>VSEDLRSRIEVLKRKVIEKVQHIQLLQKNVRAQLVDMKRLEVDIDIKIRSCRGSCSRALAREVDLKDYEDQQKQLEQVIAKDLLPSR[2x];>DNENVVNEYSSELEKHQLYIDETVNSNIPTNLRVLRSILENLRSKIQKLESDVSAQMEYCRTPCTVSCNIPVVSGKECEEIIRKGGETSEMYLIQPDSSVKPYRVYCDMNTENGGWTVIQNRQDGSVDFGRKWDPYKQGFGNVATNTDGKNYCGLPGEYWLGNDKISQLTRMGPTELLIEMEDWKGDKVKAHYGGFTVQNEANKYQISVNKYRGTAGNALMDGASQLMGENRTMTIHNGMFFSTYDRDNDGWLTSDPRKQCSKEDGGGWWYNRCHAANPNGRYYWGGQYTWDMAKHGTDDGVVWMNWKGSWYS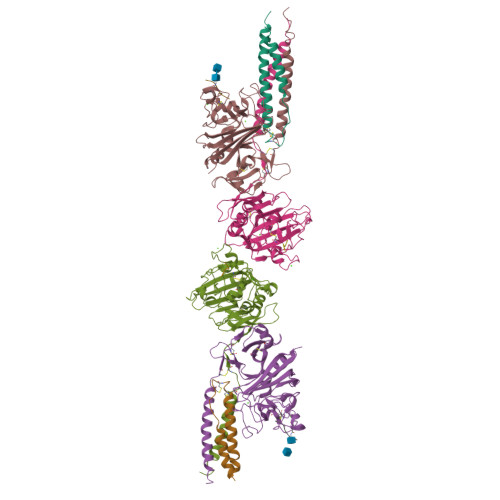MRKMSMKIRPFFP[2x];>KMLEEIMKYEASILTHDSSIRYLQEIYNSNNQKIVNLKEKVAQLEAQCQEPCKDTVQIHDITGKDCQDIANKGAKQSGLYFIKPLKANQQFLVYCEIDGSGNGWTVFQKRLDGSVDFKKNWIQYKEGFGHLSPTGTTEFWLGNEKIHLISTQSAIPYALRVELEDWNGRTSTADYAMFKVGPEADKYRLTYAYFAGGDAGDAFDGFDFGDDPSDKFFTSHNGMQFSTWDNDNDKFEGNCAEQDGSGWWMNKCHAGHLNGVYYQGGTYSKASTPNGYDNGIIWATWKTRWYSMKKTTMKIIPFNRLTIGEGQQHHLGGAKQAGDV[2x];>[2x]GHRPY;>[2x]GHRP>GASMPLKPEEHEDILNKLLDPELAQSERTEALQQLRVNYGSFVSEYNDLTKSHAHLERMKKNMEQTIKDLQHRLDEAEQIALKGGKKQLQKLEARVRELENELEAEQKRNAESVKGMRKSERRIKELTYQTED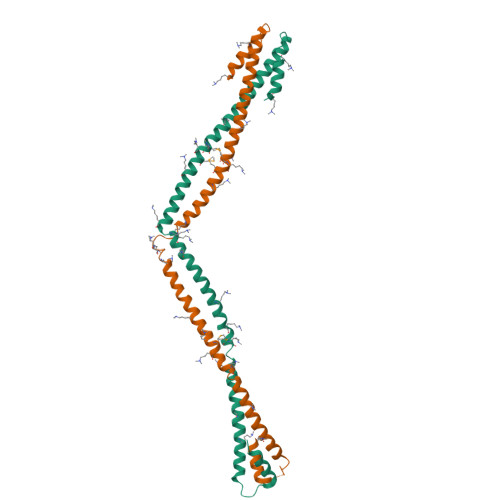LEKERDFYFGKLRNIELICQENEGENDPVLQRIVDILYATDE[4x]>[7x]XGEIAQAMKEIAKAMKEIA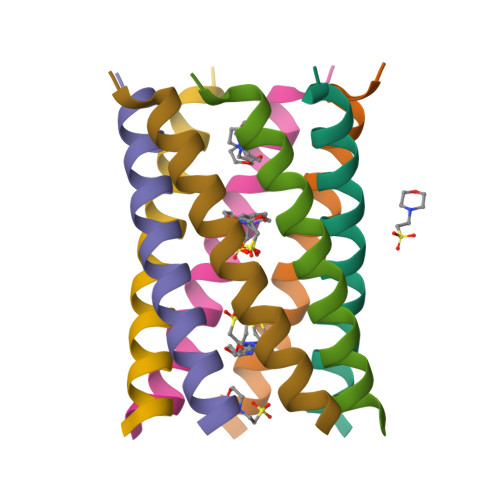WAMKEIAQAMKGX> MNGVYDVGGTDGLGPINRPADEPVFRAEWEKVAFAMFPATFRAGFRGLDEFRFGIEQMNPAEYLESPYYWHWIRTYIHHGVRTGKIDLEELERRTQYYRENPDAPLPEHEQKPELIEFVNQAVYGGLPASREVDRPPKFKEGDVVRFSTASPKGHARRARYVRGKTGTVVKHHGAYIYPDTAGNGLGECPEHLYTVRFTAQELWGPEGDPNSSVYY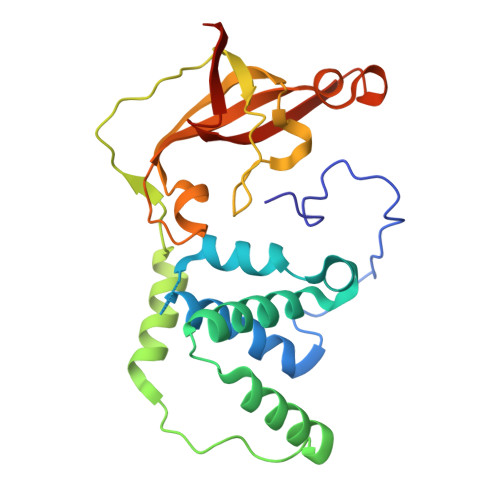DCWEPYIELVDTKAAAA> MSLVNRKQLEKMANVRFRVQEDEYVAILDALEEYHNMSENTVVEKYLKLKDINSLTDTYIDTYKKSGRNKALKKFKEYLVIEILELKNSNLTPVEKNLHFIWIGGQINDTAINYINQWKDVNSDYNVNVFYDSNAFLINTLKKTIIESASNDTLESFRENLNDPEFNHTAFFRKRMQIIYDKQQNFINYYKAQKEENPDLIIDDIVKTYLSNEYSKDIDELNAYIEESLNKVTENSGNDVRNFEEFKTGEVFN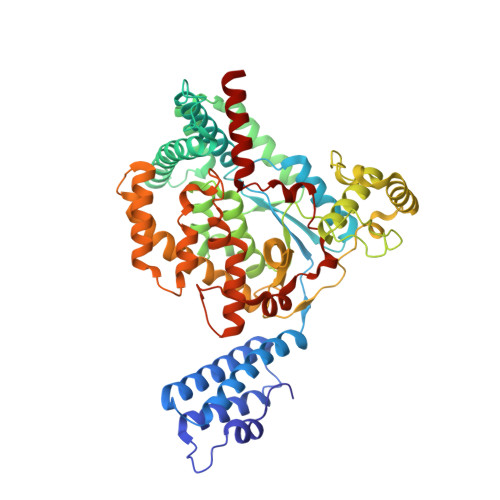LYEQELVERWNLAGASDILRVAILKNIGGVYLDVDMLPGIHPDLFKDINKPDSVKTAVDWEEMQLEAIMKHKEYIPEYTSKHFDTLDEEVQSSFESVLASKSDKSEIFLPLGDIEVSPLEVKIAFAKGSIINQALISAKDSYCSDLLIKQIQNRYKILNDTLGPIISQGNDFNTTMNNFGESLGAIANEENISFIAKIGSYLRVGFYPEANTTITLSGPTIYAGAYKDLLTFKEMSIDTSILSSELRNFEFPKVNISQATEQEKNSLWQFNEERAKIQFEEYKKNYFE SurE is one of the several proteins that gets expressed when bacterial cells are subjected to environmental stresses and in the stationary growth phase of bacteria. SurE has been shown to possess phosphatase activity and appears to be specific to nucleoside monophosphates. The StSurE protomer has a Rossmann fold like structure similar to those of its thermophilic homologs. The crystal structure of StSurE reveals that the C-terminal helices of the two protomers of the dimer are swapped.

Examination of the sequences of this segment in StSurE and PaSurE suggested that D230 and H234 of StSurE might be the key residues responsible for C-terminal helix swapping. The activity of H234A was only 5% of that of the native enzyme. The structure of H234A StSurE could not be determined by molecular replacement with acceptable scores using the Phaser program and StSurE monomer or dimer as phasing models. With this truncated model, a solution with an LLG score of 905 was obtained when two copies of the truncated protomer were placed in the asymmetric unit of the H234A StSurE. The final model of H234A StSurE consists of a dimer in the asymmetric unit with 244 residues (out of 253+14 N-terminal tag) in chain A, 252 residues in chain B, seven molecules of ethylene glycol (added as cryo-protectant), 248 water molecules and two magnesium ions. In both mutants, the two protomers of the asymmetric unit are related by a rotation of 167°. D230 OD2– H234 NE2 hydrogen bond is lost in the mutants. In chain A of H234A, D230 carboxylate is hydrogen bonded to H228 ND1 (2.90 Å). In the mutant dimers, the hinge regions of the two chains are closer (Cαs of D230s are at ∼ 5 Å). This leads to the formation of several new hydrogen bonds involving D230 in H234A (D230 O/A - D230 N/B (2.85 Å) and D230 N/A – D230 O/B (3.04 Å)). The 5% activity of H234A might be due to the presence in solution of a small fraction of molecules with a dimeric organization similar to that of the wild type enzyme.

>[2x]MRGSHHHHHHGMASMRILLSNDDGVHAPGIQTLAKALREFADVQVVAPDRNRSGASNSLTLESSLRTFTFDNGDIAVQMGTPTDCVYLGVNALMRPRPDIVVSGINAGPNLGDDVIYSGTVAAAMEGRHLGFPALAVSLNGYQHYDTAAAVTCALLRGLSREPLRTGRILNVNVPDLPLAQVKGIRVTRCGSRHPADKVIPQEDPRGNTLYWIGPPGDKYDAGPDTDFAAVDEGYVSVTPLHVDLTAASAHDVVSDWLDSVGVGTQW> GMLSLELCDDDPPEIPHATFKAMAYKEGTMLNCECKRGFRRIKSGSLYMLCTGSSSHSSWDNQCQCTSSATRSTTKQVTPQPEEQKERKTTEMQSPMQPVDQASLPGHCREPPPWENEATERIYHFVVGQMVYYQCVQGYRALHRGPAESVCKMTHGKTRWTQPQLICTGEMETSQFPGEEKPQASPEGRPESETSCL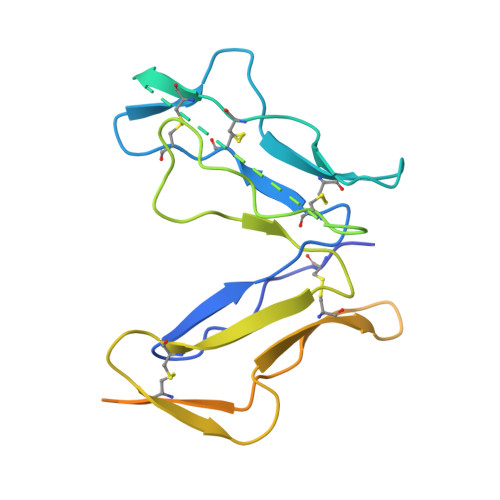VTTTDFQIQTEMAATMETSTGHHHHHH> MSTRAGDHNRQRGCCGSLADYLTSAKFLLYLGHSLSTWGDRMWHFAVSVFLVELYGNSLLLTAVYGLVVAGSVLVLGAIIGDW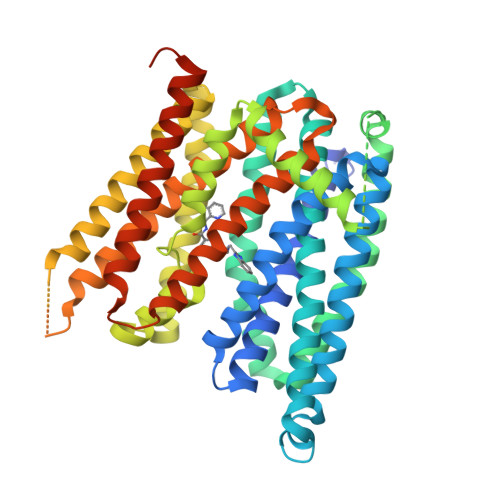VDKNARLKVAQTSLVVQNVSVILCGIILMMVFLHKHELLTMYHGWVLTSCYILIITIANIANLASTATAITIQRDWIVVVAGEDRSKLANMNATIRRIDQLTNILAPMAVGQIMTFGSPVIGCGFISGWNLVSMCVEYVLLWKVYQKTPALAVKAGLKEEETELKQLNLHKDTEPKPLEGTHLMGVKDSNIHELEHEQEPTCASQMAEPFRTFRDGWVSYYNQPVFLAGMGLAFLYMTVLGFDCITTGYAYTQGLSGSILSILMGASAITGIMGTVAFTWLRRKCGLVRTGLISGLAQLSCLILCVISVFMPGSPLDLSVSPFEDIRSRFIQGESITPTKIPEITTEIYMSNGSNSANIVPETSPESVPIISVSLLFAGVIAARIGLWSFDLTVTQLLQENVIESERGIINGVQNSMNYLLDLLHFIMVILAPNPEAFGLLVLISVSFVAMGHIMYFRFAQNTLGNKLFACGPDAKEVRKENQANTSVVALEVLFQG>[2x]MEGERMNAFPSTMMDEELNLWDFLERAAALFGRKEVVSRLHTGEVHRTTYAEVYQRARRLMGGLRALGVGVGDRVATLGFNHFRHLEAYFAVPGMGAVLHTANPRLSPKEIAYILNHAEDKVLLFDPNLLPLVEAIRGELKTVQHFVVMDEKAPEGYLAYEEALGEEADPVRVPERAACGMAYTTGTTGLPKGVVYSHRALVLHSLAASLVDGTALSEKDVVLPVVPMFHVNAWCLPYAATLVGAKQVLPGPRLDPASLVELFDGEGVTFTAGVPTVWLALADYLESTGHRLKTLRRLVVGGSAAPRSLIARFERMGVEVRQGYGLTETSPVVVQNFVKSHLESLSEEEKLTLKAKTGLPIPLVRLRVADEEGRPVPKDGKALGEVQLKGPWITGGYYGNEEATRSALTPDGFFRTGDIAVWDEEGYVEIKDRLKDLIKSGGEWISSVDLENALMGHPKVKEAAVVAIPHPKWQERPLAVVVPRGEKPTPEELNEHLLKAGFAKWQ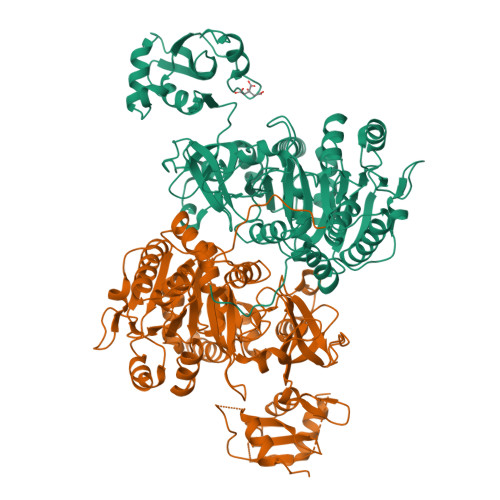LPDAYVFAEEIPRTSAGKFLKRALREQYKNYYGGA> DSRAVPTPAAWELGKKS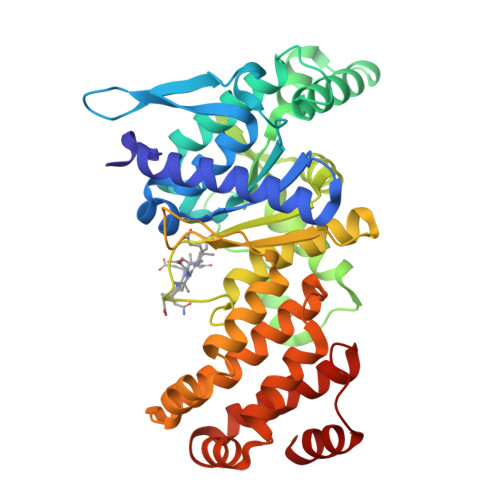AELLITRYTQDHGEWPTSFGLTAWGTSNMRTGGDDIAQALALIGVQPVWDMASRRVTGYEIVPPAKLARPRVDVTLRISGFFRDAFPEQIALFDKAVRAVGALDEDVEDNPIAARMKAEQARLVAGGADPQTAERRAGYRVFGSKPGAYGAGLQALIDENGWAGRNDLAEAWLVWGGYAYGAGEEGQAERGLLEERLRSVQAVVQNQDNREHDLLDSDDYYQFEGGMAATVESLTGAMPSVYHNDHSRPEKPVIRALEEELSRVVRGRAANPKWIAGVMRHGYKGAAEIAATVDYLFAFAATTGKVGNHHFEAVYQAYIADRAVHDFMAEKNPAALAETAAKLNEAIERGFWTPRSNSARFELENLS>[3x]MRDIDSVMRLAPVMPVLVIEDIADAKPIAEAL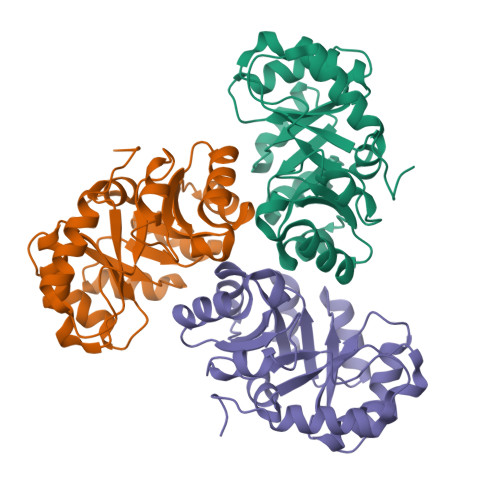VAGGLNVLEVTLRTPCALEAIKIMKEVPGAVVGAGTVLNAKMLDQAQEAGCEFFVSPGLTADLGKHAVAQKAALLPGVANAADVMLGLDLGLDRFKFFPAENIGGLPALKSMASVFRQVRFCPTGGITPTSAPKYLENPSILCVGGSWVVPAGKPDVAKITALAKEASAFKRAAVA>GSGAMDELLRRAVPPTPAYELREKTPAPAEGQCADFVSFYGGLAETAQRAELLGRLARGFGVDHGQVAEQSAGVLHLRQQQREAAVLLQAEDRLRYALVPRYRGLFHHISKLDGGVRFLVQLRADLLEAQALKLVEGPDVREMNGVLKGMLSEWFSSGFLNLERVTWHSPCEVLQKISEAEAVHPVKNWMDMKRRVGPYRRCYFFSHCSTPGEPLVVLHVALTGDISSNIQAIVKEHPPSETEEKNKITAAIFYSISLTQQGLQGVELGTFLIKRVVKELQREFPHLGVFSSLSPIPGFTKWLLGLLNSQTKEHGRNELFTDSECKEISEITGGPINETLKLLLSSSEWVQSEKLVRALQTPLMRLCAWYLYGEKHRGYALNPVANFHLQNGAVLWRINWMADVSL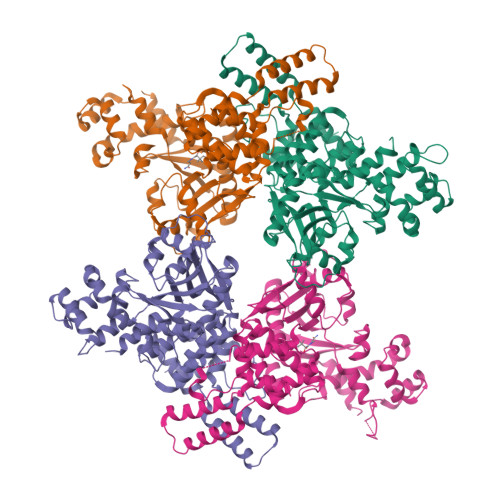RGITGSCGLMANYRYFLEETGPNSTSYLGSKIIKASEQVLSLVAQFQKNSKL[8x]>SNAMSQFMNLEGKVALVTGASRGIGKAIAELLAERGAKVIGTATSESGAQAISDYLGDNGKGMALNVTNPESIEAVLKAITDEFGGVDILVNNAGITRDNLLMRMKEEEWSDIMETNLTSIFRLSKAVLRGMMKKRQGRIINVASVVGTMGNAGQANYAAAKAGVIGFTKSMAR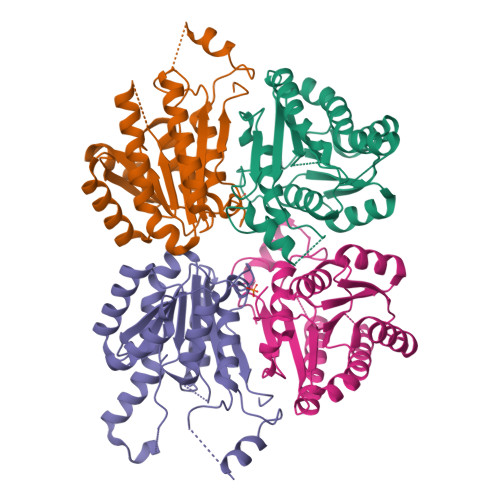EVASRGVTVNTVAPGFIETDMTKALNDEQRTATLAQVPAGRLGDPREIASAVAFLASPEAAYITGETLHVNGGMYMI[4x]> DVYTDHGDLYNTPVRMLVVAGAKFKEALKPWLTWKAQKGFYLDVHYTDEAEVGTTNASIKAF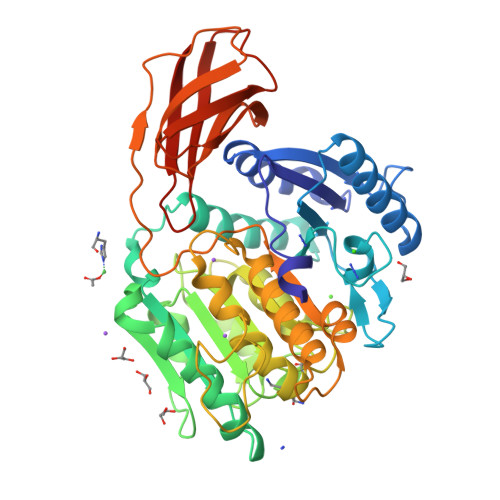IHKKYNDGLAASAAPVFLALVGDTDVISGEKGKKTKKVTDLYYSAVDGDYFPEMYTFRMSASSPEELTNIIDKVLMYEKATMPDKSYLEKVLLIAGADYSWNSQVGQPTIKYGMQYYYNQEHGYTDVYNYLKAPYTGCYSHLNTGVSFANYTAHGSETAWADPLLTTSQLKALTNKDKYFLAIGNCCITAQFDYVQPCFGEVITRVKEKGAYAYIGSSPNSYWGEDYYWSVGANAVFGVQPTFEGTSMGSYDATFLEDSYNTVNSIMWAGNLAATHAGNIGNITHIGAHYYWEAYHVLGDGSVMPYRAMPKTNTYTLPASLPQNQASYSIQASAGSYVAISKDGVLYGTGVANASGVATVSMTKQITENGNYDVVITRSNYLPVIKQIQVGEPHHHHHH> MDHRTSIAQALVDRIAQQMDGSQPDEYFNNLYGNVSRQTYKF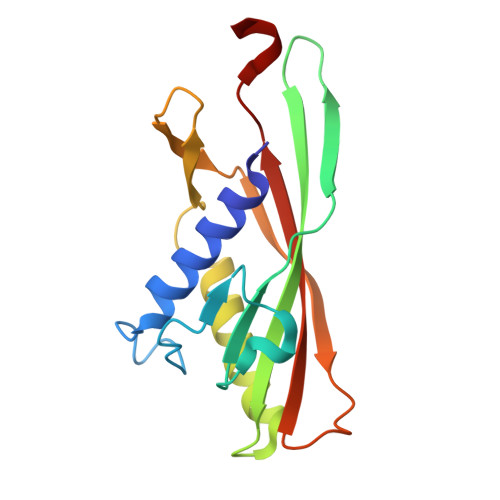EEIREFPYVAVHIGTETGQYLPSGQQWMFLELPILVYDKEKTDIQEQLEKLVADIKTVIDTGGNLEYTVSKPNGSTFPCEATDMSITSVSTDEGLLAPYGLAEINVTVRYQPPRRSLRR>MDITEKLRLITRNAEEVVTEEELRQLIETKEKPRAYVGYEPSGEIHLGHMMTVQKLMDLQEAGFEIIVLLADIHAYLNEKGTFEEIAEVADYNKKVFIALGLDESRAKFVLGSEYQLSRDYVLDVLKMARITTLNRARRSMDEVSRRKEDPMVSQMIYPLMQALDIAHLGVDLAVGGIDQRKIHMLARENLPRLGYSSPVCLHTPILVGLDGQKMSSSKGNYISVRDPPEEVERKIRKAYCPAGVVEENPILDIAKYHILPRFGKIVVERDAKFGGDVEYASFEEL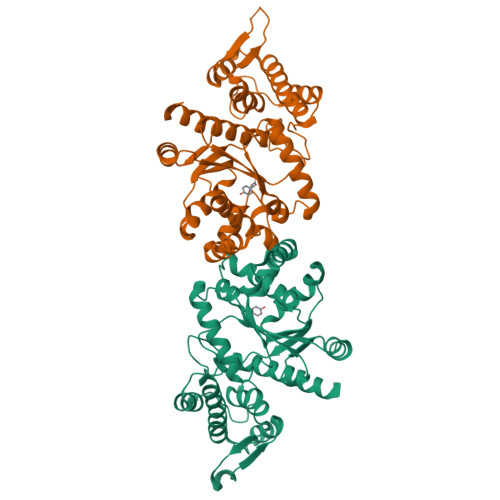AEDFKSGQLHPLDLKIAVAKYLNMLLEDARKRLGVSV[2x]>[3x]SNAMDAYEIIQYIGDA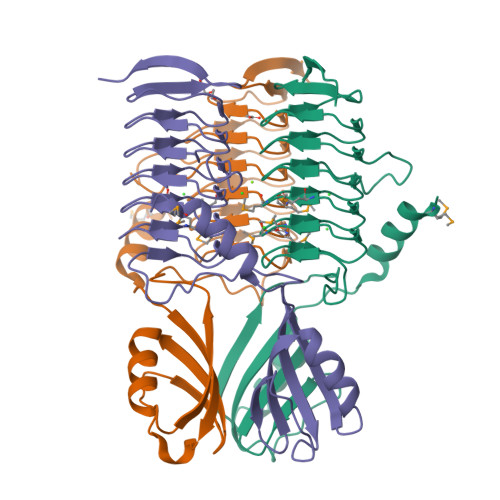KKQTLVKVTLKGQLKEVTFPETIKVFNNCKTGTLFGDWADVKPFLEANKEKIEDYVVENDARNSAIPFLDLKDINARIEPGALIREKVEIGDQAVIMMGAILNIGAVVGAGTMIDMGAVLGGRATVGKHCHIGAGTVLAGVIEPPSAAPVVIENEVVIGANAVVLEGVRVGEGAVVAAGAVVVEDVPAHTVVAGVPAKVIKQIDDKTKSKTEILEELRKL>[4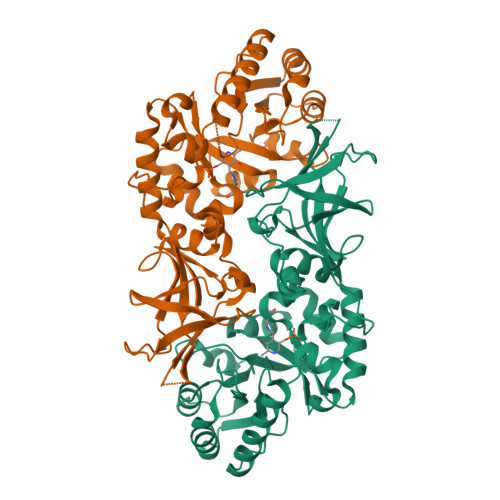x]MNLLTTKIDLDAIAHNTRVLKQMAGPAKLMAVVKANAYNHGVEKVAPVIAAHGADAFGVATLAEAMQLRDIGISQEVLCWIWTPEQDFRAAIDRNIDLAVISPAHAKALIETDAEHIRVSIKIDSGLHRSGVDEQEWEGVFSALAAAPHIEVTGMFTHLACADEPENPETDRQIIAFRRALALARKHGLECPVNHVCNSPAFLTRSDLHMEMVRPGLAFYGLEPVAGLEHGLKPAMTWEAKVSVVKQIEAGQGTSYGLTWRAEDRGFVAVVPAGYADGMPRHAQGKFSVTIDGLDYPQVGRVCMDQFVISLGDNPHGVEAGAKAVIFGENGHDATDFAERLDTINYEVVCRPTGRTVRAYV2-phenyl-4-[[(3~{S})-piperidin-3-yl]amino]-1~{H}-indole-7-carboxamide | C20 H22 N4 O | 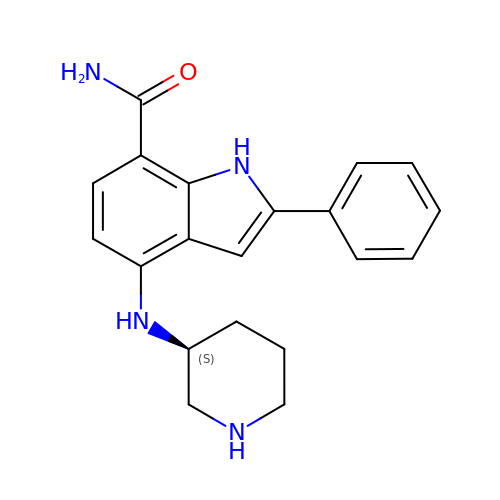AQEDGKFVSWOMSY-AWEZNQCLSA-N> RARIERARSIEG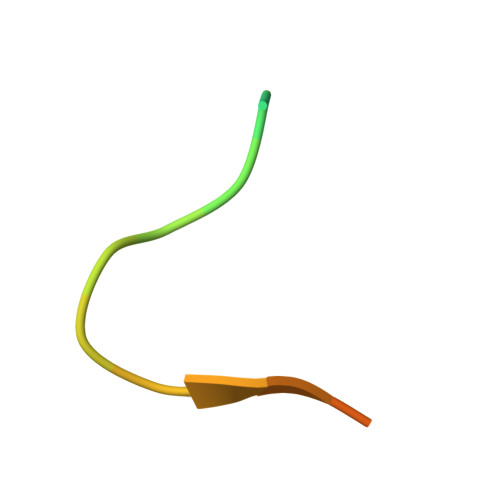AVQVSKGTG> CGCTATAATGCG;>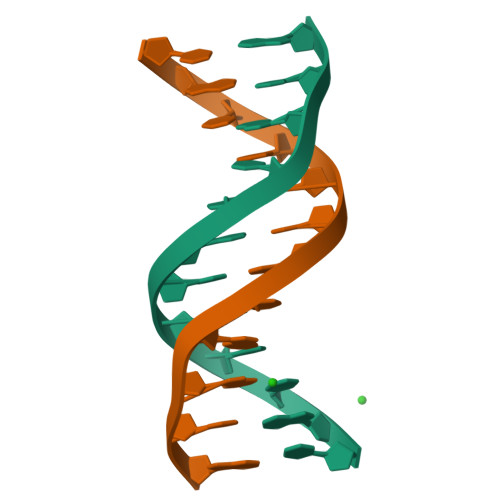 CGCATTATAGCG>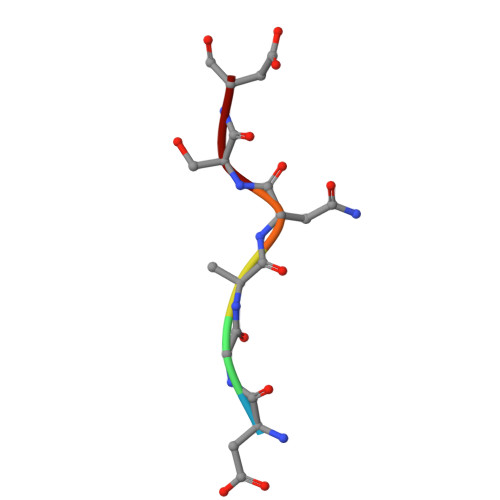 DGANSD> MAHHHHHHSAALEVLFQGPLAPYEIIVSEDSEHLGKSIGELNVWHQTGATIVAIEHEGKFIVSPGPFSVIEQGDHIFFVGDEDVYARMKTYFNLRM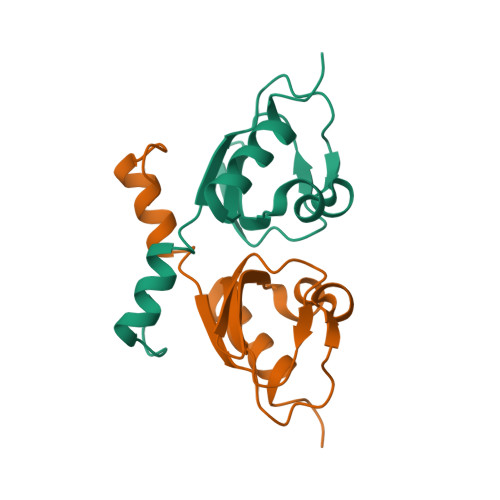GL> SMDMPVERILEAELAVEPKTESYGDMNMENSTNDPVTNICHAADKQLFTLVEWAKRIPHFSDLTLEDQVILLRAGWNELLIASFSHRSVSVQDGIL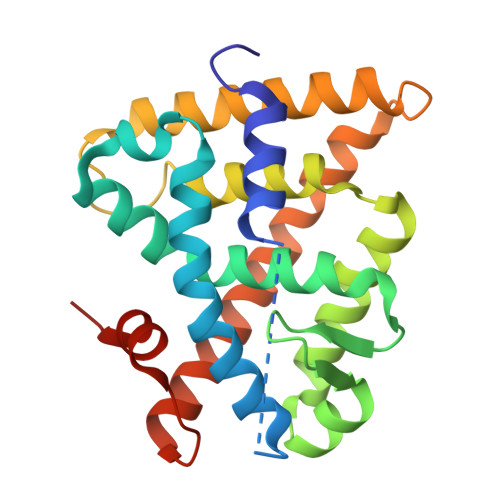LATGLHVHRSSAHSAGVGSIFDRVLTELVSKMKDMQMDKSELGCLRAIVLFNPDAKGLSNPSEVETLREKVYATLEAYTKQKYPEQPGRFAKLLLRLPALRSIGLKCLEHLFFFKLIGDTPIDTFLMEMLETPLQIT>TTIVSVRRNGHVVIAGDGQATLGNTVMKGNVKKVRRLYNDKVIAGFAGGTADAFTLFELFERKLEMHQGHLVKAAVELAKDWRTDRMLRKLEALLAVADETASLIITGNGDVVQPENDLIAIGSGGPYAQAAARALLENTELSAREIAEKALDIAGDICIYTNHFHTIEELSYKA[4x];>[2x]MSEMTPREIVSELDKHIIGQDNAKRSVAIALRNRWRRMQLNEELRHEVTPKNILMIGPTGVGKTEIARRLAKLANAPFIKVEATKF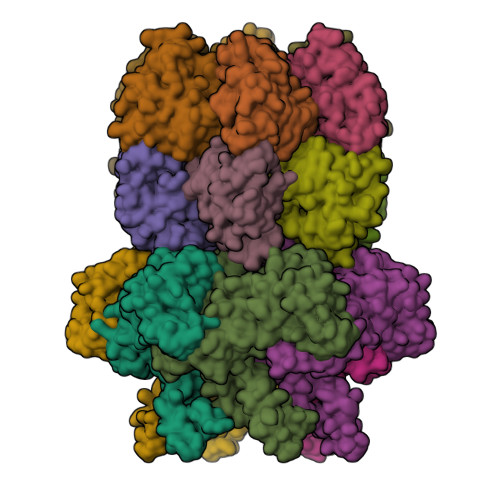TEVGYVGKEVDSIIRDLTDAAVKMVRVQAIEKNRYRAEELAEERILDVLIPPAKNNWGQTEQQQEPSAARQAFRKKLREGQLDDKEIEIDLAAAPMGVEIMAPPGMEEMTSQLQSMFQNLGGQKQKARKLKIKDAMKLLIEEEAAKLVNPEELKQDAIDAVEQHGIVFIDEIDKICKRGESSGPDVSREGVQRDLLPLVEGCTVSTKHGMVKTDHILFIASGAFQIAKPSDLIPELQGRLPIRVELQALTTSDFERILTEPNASITVQYKALMATEGVNIEFTDSGIKRIAEAAWQVNESTENIGARRLHTVLERLMEEISYDASDLSGQNITIDADYVSKHLDALVADEDLSRFIL Microrchidia CW-type zinc finger proteins (MORCs) are a family of transcriptional regulators conserved in eukaryotes. We recently showed that human MORC2 is necessary, in conjunction with the human silencing hub (HUSH), for silencing of transgenes integrated at chromatin loci with histone H3 trimethylated at lysine 9 H3K9me3. MORC2 is a 1032-amino acid protein predicted to contain several functional domains including an N-terminal GHKL-type ATPase module with a coiled-coil insertion (CC1). Here we report the biochemical and cellular activities of MORC2 variants, alongside structures of wild-type and neuropathic variant forms of a MORC2 fragment comprising the GHKL-type ATPase module and CW domain.

The effect of T424R on the crystal structure of MORC2 is more subtle. The backbone structures of wild-type and T424R are essentially identical, including in the loop that contains the mutation. The arginine sidechain in the mutant does make an additional salt bridge across the dimer interface, with Glu27 from the other protomer. Moreover, the buried surface area at the dimer interface is actually decreased upon the T424R mutation (2527 Å2 buried per protomer versus 2778 Å2 in wild type). The contribution of the mutant Arg424 sidechain to the dimer interface, and its position just three residues away from a key active site residue Lys427, can be expected to alter the ATP-dependent dimerization dynamics of MORC2. Indeed, we found that the T424R variant forms a mixture of monomers and dimers in the presence of AMPPNP, and shows an elevated rate of ATP hydrolysis. This suggests that T424R dimers may form and dissociate more rapidly than in the wild type. Conversely, T424R (which has increased ATPase activity in vitro) was significantly less efficient at GFP reporter repression than wild-type at both loci.

>GPRMAFTNYSSLNRAQLTFEYLHTNSTTHEFLFGALAELVDNARDADATRIDIYAERREDLRGGFMLCFLDDGAGMDPSDAASVIQFGKSAKRTPESTQIGQYGNGLKSGSMRIGKDFILFTKKEDTMTCLFLSRTFHEEEGIDEVIVPLPTWNARTREPVTDNVEKFAIETELIYKYSPFRTEEEVMTQFMKIPGDSGTLVIIFNLKLMDNGEPELDIISNPRDIQMAETSPEGTKPERRSFRAYAAVLYIDPRMRIFIHGHKVQTKRLSCCLYKPRMYKYTSSRFKTRAEQEVKKAEHVARIAEEKAREAESKARTLEVRLGGDLTRDSRVMLRQVQNRAITLRREADVKKRIKEAKQRALKEPKELNFVFGVNIEHRDLDGMFIYNCSRLIKMYEKVGPQLEGGMACGGVVGVVDVPYLVLEPRHNKQDFADAKEYRHLLRAMGEHLAQYWKDIAIAQRGIIKFWDEFGYLSANWNQPPSSELRYKRRRAMEIPTTIQCDLCLKWRTLPFQLSSVEKDYPDTWVCSMNPDPEQDRCEASEQKQKVPLGTFRKDMKTQEEKQKQLTEKIRQQQEKLEALQKTTPIRSQADLKKLPLEVTTRPST[2x]PHOSPHORYLATED 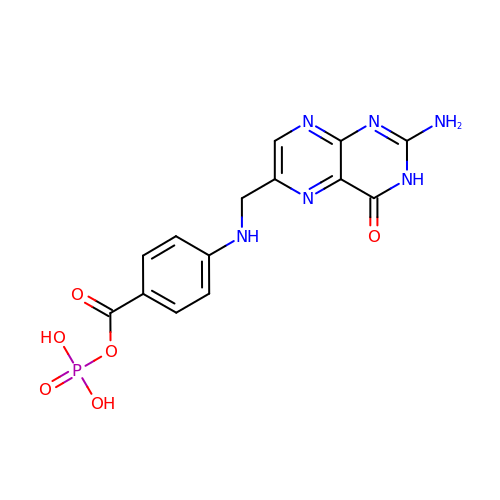DIHYDROPTEROATE | C14 H13 N6 O6 P | DNKVHXNVVYQUDC-UHFFFAOYSA-N> AHMTNGWVIGVDPDIGGAIAVLSPDGSSQVFDNPFVHIVVSEVIRKRLDTKSIIELLRGLDAPPGTTAYIEKSSPFPTDGKQGWWSTGFSYGLWIASLVASGFSVVPVASQTWKAYFGLMRSETPKDDSRQAASILFPDKDQSLKLKKHHGRAEALLLAAYGKGLVLPSGKFSKTSV

Recently, mutational screening analysis identified the chloroplast-localized HJ resolvase MOC1 that is essential for chloroplast nucleoid segregation in Chlamydomonas reinhardtii and Arabidopsis thaliana. MOC1 exhibits dimerization and an RNaseH fold, belonging to the retroviral integrase superfamily. Moreover, we characterize a base recognition loop (BR loop) that protrudes into the junction and disrupts the C–G base pairs at the crossover. Residue D183 from the BR loop recognizes the cytosine, determining the cytosine-dependent HJ resolution.

In this study, we determine the crystal structures of HJ-free Zea mays MOC1 (ZmMOC1), Nicotiana tabacum MOC1 (NtMOC1), and HJ-bound NtMOC1 at resolutions of 2.5 Å, 2.0 Å, and 2.5 Å, respectively. We first determined the crystal structure of HJ-free ZmMOC1 (T107-V280) via iodide-based single-wavelength anomalous diffraction (I-SAD) at a refined resolution of 2.5 Å and the structure of a quadruple mutant NtMOC1 (N108-S275, I112V/Q162K/E235Q/239Q) at a 2.0 Å resolution. Structural alignment of NtMOC1 with ZmMOC1 revealed a similar fold with an RMSD value of 0.919 Å.>MGFTEETVRFRLDDTDKQEISKTLTSVYRSLEEKGYNPINQIIGYVLSGDPAYIPRYNDARNQIRK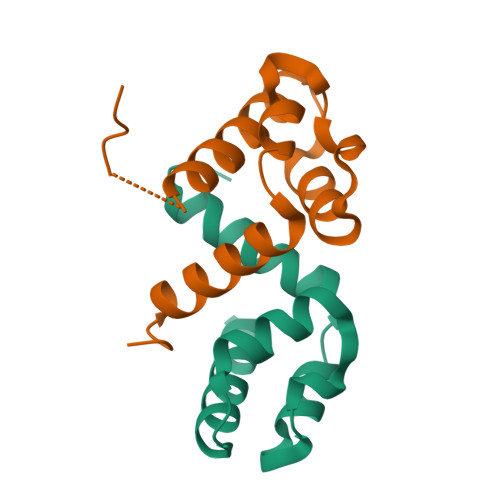HERDEIIEELVRYYLKGNGIDL[2x]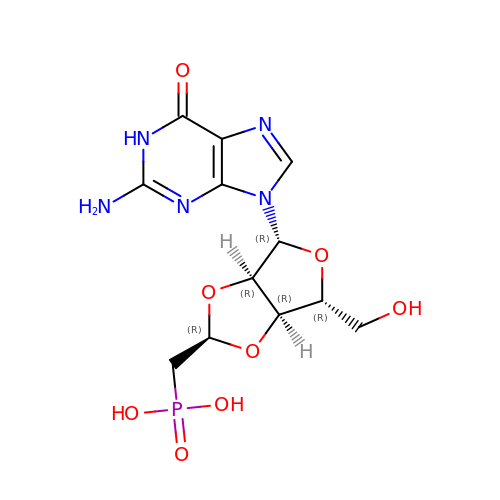((2R,4R,6R,6AS)-4-(2-AMINO-6-OXO-1,6-DIHYDROPURIN-9-YL)-6-(HYDROXYMETHYL)-TETRAHYDROFURO[3,4-D][1,3]DIOXOL-2-YL)METHYLPHOSPHONIC ACID | C12 H16 N5 O8 P | HYAPEMYRVFIHDJ-QWEIRQIHSA-N> GSKKRQRFVDKNGRCNVQHGNLGSERAETLMFSEHAVISMRDGKLTLMFRVGNLRNSHMVSAQIRCKLLKSRQTPEGEFLPLDQLELDVGFSTGADQLFLVSPLTICHVIDAKSPFYDLSQRSMQTEQFEVVVILEGIVETTGMTCQARTSYTEDEVLWGHRFFPVISLEEGFFKVDYSQFHATFEVPTPPYSVKEQE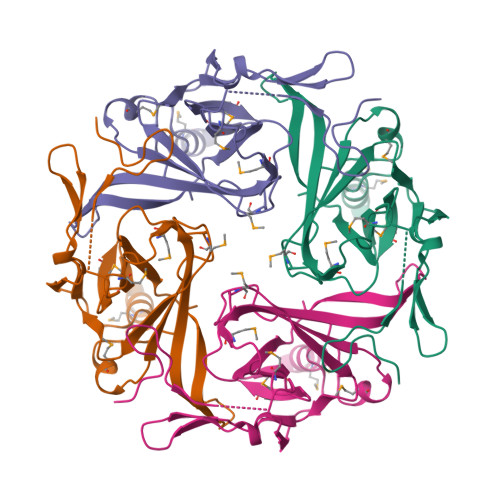EMLLMSSPL>[2x]TSMDPSSPNYDKWEMERTDITMKHKLGGGQYGEVYEGVWKKYSLTVAVKTLKEDTMEVEEFLKEAAVMKEIKHPNLVQLLGVCTREPPFYIIIEFMTYGNLLDYLRECNRQEVN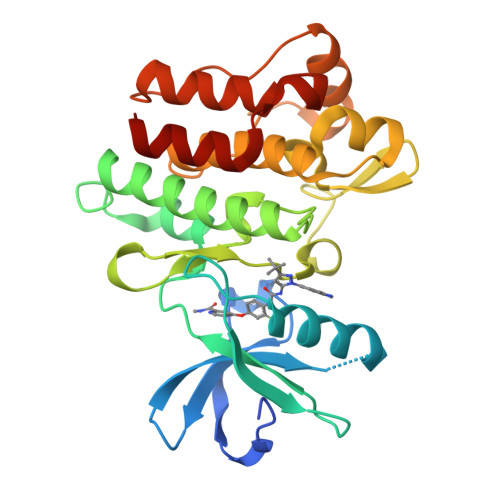AVVLLYMATQISSAMEYLEKKNFIHRDLAARNCLVGENHLVKVADFGLSRLMTGDTYTAHAGAKFPIKWTAPESLAYNKFSIKSDVWAFGVLLWEIATYGMSPYPGIDLSQVYELLEKDYRMERPEGCPEKVYELMRACWQWNPSDRPSFAEIHQAFETMFQE>GMTISRNYDQEIKDTAGHKYAYNFDFDVMHPFMVRAFTPFFRPGNLLELGSFKGDFTSRLQEHFNDITCVEASEEAISHAQGRLKDGITYIHSRFEDAQLPRRYDNIVLTHVLEHIDDPVALLKRINDDWLAEGGRLFLVCPNANAVSRQIAVKMGIISHNSAVTEAEFAHGHRCTYALDTLERDASRAGLQVTYRSGIFFKALANFQWDQILQTDILSK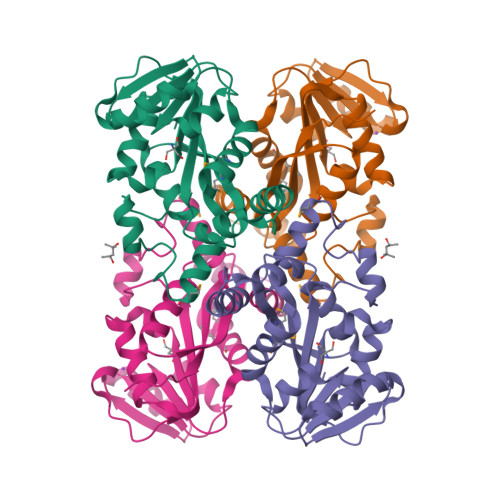EYLDGCYQLGQQYPDLCASIFLLCEKGINQ[2x]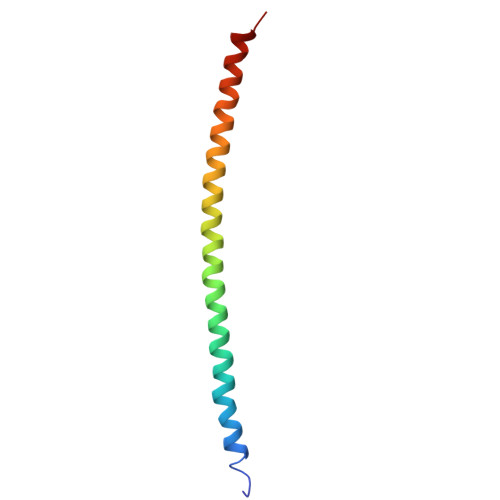> LAAKEAKLRDLEDSLARERDTSRRLLAEKEREMAKMRARMQQQLDEYQELLDIKLALDMEIHAYRKLLEGEEER>TTSAEKNTCQLYIQTDHLFFKYYGTREAVIAQISSHVKAIDTIYQTTDFSGIRQISFMVKRIRINTTADEKDPTNPFRFPNIGVEKFLELNSEQNHDDYCLAYVFTDRDFDDGVLGLAWVGAPSGSSGGICEKSKLYSDGKKKSLNTGIITVQNYGSHVPPKVSHITFAHEVGHNFGSPHDSGTECTPGESKNLGQKENGNYIMYARATSGDKLNNNKFSLCSIRQISQVLEKKRNNCFVES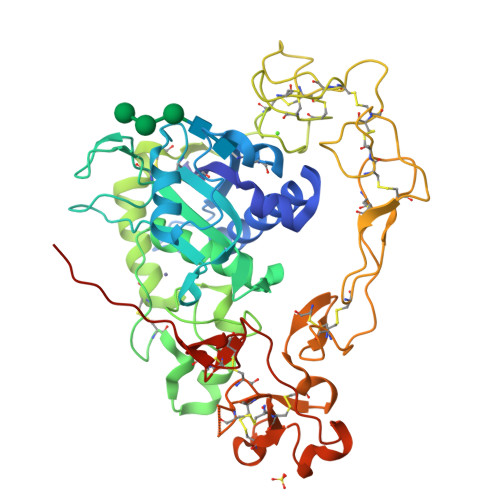GQPICGNGMVEQGEECDCGYSDQCKDECCFDANQPEGRKCKLKPGKQCSPSQGPCCTAQCAFKSKSEKCRDDSDCAREGICNGFTALCPASDPKPQFTDCNRHTQVCINGQCAGSICEKYGLEECTCASSDGKDDKELCHVCCMKKMDPSTCASTGSVQWSRHFSGRTITLQPGSPCNDFRGYCDVFMRCRLVDADGPLGGHHHHHH[4x]TETRAETHYLAMMONIUM ION | C8 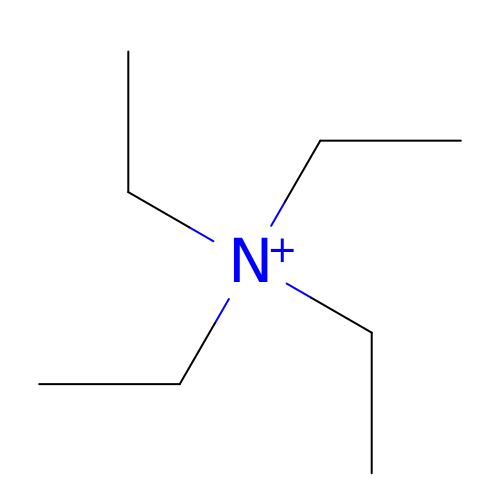H20 N | CBXCPBUEXACCNR-UHFFFAOYSA-N>[4x]MNANLFARLFDKLDDPHKLAIETAAGDKISYAELVARAGRVANVLVARGLQVGDRVAAQTEKSVEALVLYLATVRAGGVYLPLNTAYTLHELDYFITDA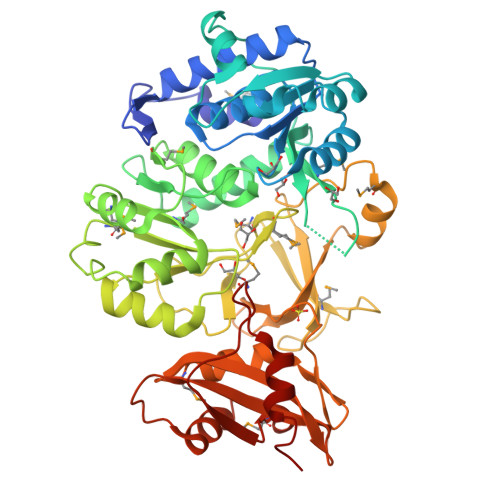EPKIVVCDPSKRDGIAAIAAKVGATVETLGPDGRGSLTDAAAGASEAFATIDRGADDLAAILYTSGTTGRSKGAMLSHDNLASNSLTLVDYWRFTPDDVLIHALPIYHTHGLFVASNVTLFARGSMIFLPKFDPDKILDLMARATVLMGVPTFYTRLLQSPRLTKETTGHMRLFISGSAPLLADTHREWSAKTGHAVLERYGMTETNMNTSNPYDGDRVPGAVGPALPGVSARVTDPETGKELPRGDIGMIEVKGPNVFKGYWRMPEKTKSEFRDDGFFITGDLGKIDERGYVHILGRGKDLVITGGFNVYPKEIESEIDAMPGVVESAVIGVPHADFGEGVTAVVVRDKGATIDEAQVLHGLDGQLAKFKMPKKVIFVDDLPRNTMGKVQKNVLRETYKDIYK>GAMIHQRLRPFPDHFLWGSASAAYQIEGAWNEDGKGLSVWDVFTKIPGKTFKGSNGDIAVDHYHRFKEDVALMAEMGLKAYRFSVSWPRIFPQGRGEANESGLRFYDDLINELLAHDIEPVLTLYHWDLPQALMDEYGGFESRRIIEDFNAYCVTLYKRYGGRVKYWVSLNEQNYNFNHGFITAMHPPGVKDRKRFYEANHIAFLANAKAIDSFRRYVPDGKIGPSFAYSPAYPLSSRPDDILAFENAEEFTNYWWLDMYCRGTYPDIPLKYLKEKGWAPTIEDGDMELLAKGKPDFVGVNYYQTITYEMNPLDGVSEGKMNTTGQKGSNQETGMPGLYKTKRNPHLETSNWDWAIDPIGLRIGLRRISSRYGLPLFITENGLGEFDKVENDGTIHDDYRIAYLRAHLEQCRQ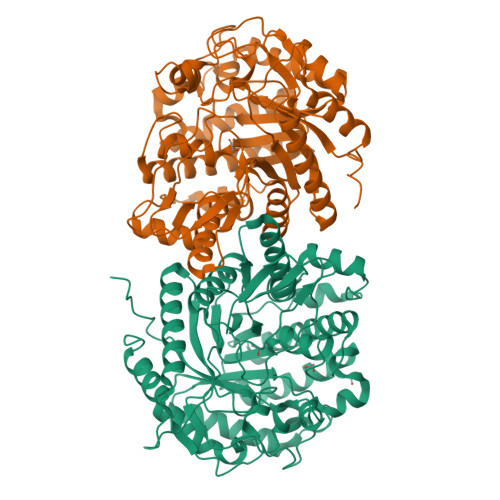ALNDGVDLIGYCSWSFTDLLSWLNGYQKRYGFVYINRDEENVKDLKRIKKDSFYWYQNVIQTNGEEL[4x]>[3x]NPRWEQ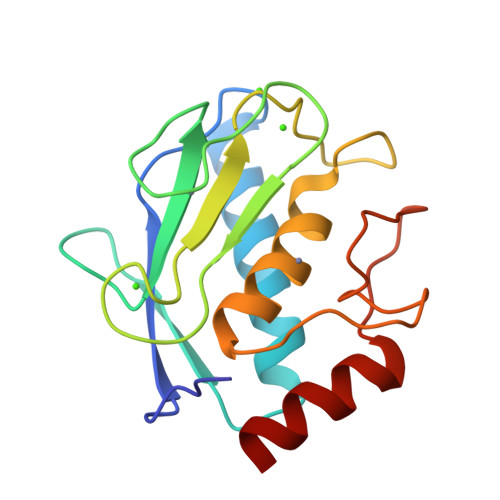THLTYRIENYTPDLPRADVDHAIEKAFQLWSNVTPLTFTKVSEGQADIMISFVRGDHRDNSPFDGPGGNLAHAFQPGPGIGGDAHFDEDERWTNNFREYNLHRVAAHELGHSLGLSHSTDIGALMYPSYTFSGDVQLAQDDIDGIQAIYG>[2x]DSDDRVTPPAEPLDRMPDPYRPSYGRAETVVNNYIRKWQQVYSHRDGRKQQMTEEQREWLSYGCVGVTWVNSGQYPTNRLAFASFDEDRFKNELKNGRPRSGETRAEFEGRVAKESFDEEKGFQRAREVASVMNRALENAHDES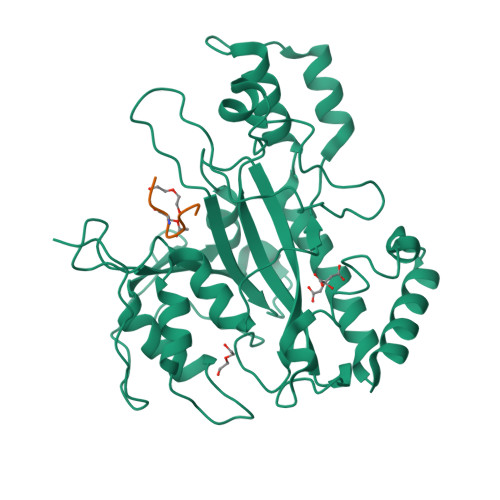AYLDNLKKELANGNDALRNEDARSPFYSALRNTPSFKERNGGNHDPSRMKAVIYSKHFWSGQDRSSSADKRKYGDPDAFRPAPGTGLVDMSRDRNIPRSPTSPGEGFVNFDYGWFGAQTEADADKTVWTHGNHYHAPNGSLGAMHVYESKFRNWSEGYSDFDRGAYVITFIPKSWNTAPDKVKQGWP;>[2x]DIPIGSKMT>[2x]ERRRGLTDPEMAAVILKALPEAPLDGNNKMGYFVTPRWKRLTEYEALTVYAQPNADWIAGGLDWGDWTQKFHGGRPSWGNETTELRTVDWFKHRDPLRRWHAPYVKDKAEEWRYTDRFLQGYSADGQIRAMNPTWRTSSCNRYWGAFLFNEYGLFNAHSQGAREALSDVTRVSLAFWGFDKIDIAQMIQLERGFLAKIVPGFDESTAVPKAEWTNGEVYKSARLAVEGLWQEVFDWNESAFSVHAVYDALFGQFVRREFFQRLAPRFGDNLTPFFINQAQTYFQIAKQGVQDLYYNCLGDDPEFSDYNRTVMRNWTGKWLEPTIAALRDFMGLFAKLPAGTTDKEEITASLYRVVDDWIEDYASAIDFKADRDQIVKAVLAGLK;>AANRAPTSVNAQEVHRWLQSFNWDFKNNRTKYATKYKMANETKEQFKLIAKEYARMEAVKDERQFGSLQVALTRLNAGVRVHPKWNETMKVVSNFLEVGEYNAIAATGMLWDSAQAAEQKNGYLAQVLDEIRHTHQCAYVNYYFAKNGQDPAGHNDARRTRTIGPLWKGMKRVFSDGFISGDAVECSLNLQLVGEACFTNPLIVAVTEWAAANGDEITPTVFLSIETDELRHMANGYQTVVSIANDPASAKYLNTDLNNAFWTQQKYFTPVLGMLFEYGSKFKVEPWVKTWDRWVYEDWGGIWIGRLGKYGVESPRSLKDAKQDAYWAHHDLYLLAYALWPTGFFRLALPDQ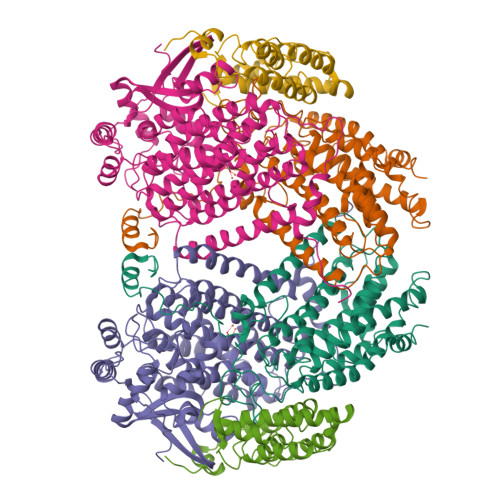EEMEWFEANYPGWYDHYGKIYEEWRARGCEDPSSGFIPLMWFIENNHPIYIDRVSQVPFCPSLAKGASTLRVHEYNGEMHTFSDQWGERMWLAEPERYECQNIFEQYEGRELSEVIAELHGLRSDGKTLIAQPHVRGDKLWTLDDIKRLNCVFKNPVKAF[2x];>[2x]LGIHSNDTRDAWVNKIAHVNTLEKAAEMLKQFRMDHTTPFRNSYELDNDYLWIEAKLEEKVAVLKARAFNEVDFRHKTAFGEDAKSVLDGTVAKMNAAKDKWEAEKIHIGFRQAYKPPIMPVNYFLDGERQLGTRLMELRNLNYYDTPLEELRKQRGVRVVH> MHHHHHHHHSSGLVPRGSAMGSSGLSIIPPESLYKKLSNRSSSNQHLNNVTWPGGTSETPRGWVFPNNGRRLRIGVPDRASFKEFVSRLDGSNKVQGYAIDVFEAAVKLISYPVPHEFVLFGDGL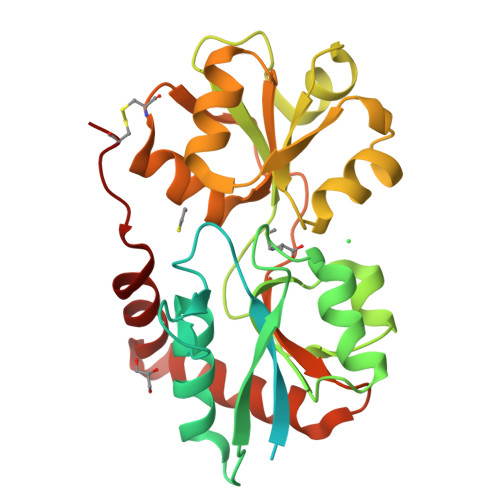KNPNFNEFVNNVTIGVFDAVVGDIAIVTKRTRIVDFTQPYIESGLVVVAPVGTPIRGVDTLISSSGRVGFQVGSYAENYMIDELNIARSRLVPLGSPKEYAAALQNGTVAAIVDERPYVDLFLSEFCGFAIRGQEFTRSGWGFAFPRDSPLAIDMSTAILGLSETGQLQKIHDKWLSRSNCSN> GSHMADPDVLTEVPAALKRLAKYVIRGFYGIEHALALDILIRNSCVKEEDMLELLKFDRKQLRSVLNNLKGDKFIKCRMRVETAADGKTTRHNYYFINYRTLVNVVKYKLDHMRRRIETDERDSTNRASFKCPVCSSTFTDLEANQLFDPMTGTFRCTFCHTEVEEDESAMPKKDARTLLARFNEQIEPIYALLRETEDVNLAYEIL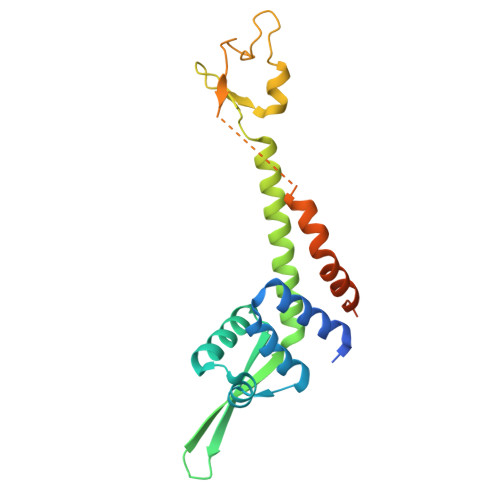EPEPTEIPALKQS Structural and functional analysis identified IPO as a member of the JRL family but with a different tetrameric association. The monomeric IPO from residues 1 to 154 shows a typical β-prism fold found in the JRL family, with 12 β-sheets (β3-β14) and 2 additional short, extended, N-terminal β-strands (β1-β2). Four IPO protomers form a compact tetrameric association by swapping their extended N termini from residues 1 to 10. Thus, the wound-inducible protein IPO from sweet potato has versatile carbohydrate binding properties and might play a role in plant defense.

IPO–Me-Man belongs to an orthorhombic space group C2221. The Matthew coefficient and solvent content for IPO–Me-Man had a reasonable value of 2.21 Å3/Da and 44.4% for 2 molecules in an asymmetric unit. Although only 2 IPO molecules were built in the IPO–Me-Man complex, the other 2 IPO molecules could be generated by symmetric operation (X, -Y, -Z) and resulted in a tetrameric association. In the structure of IPO–Me-Man, two IPO protomers were built, and only one Me-Man molecule could be observed in chain A. The temperature factor of Me-Man in the structure of IPO–Me-Man is 66.5 Å2, which is higher than that of Me-Glc, with 34.5 Å2. This phenomenon might indicate that only a few Me-Man molecules bound to IPO proteins in IPO–Me-Man, which resulted in a higher temperature factor. Nine hydrogen bonds are formed by the residues Gly21, Tyr97, Gly141, Trp142, Tyr143, and Asp145 of IPO and the atoms O1, O3, O4, O5 and O6 of Me-Man. The atom C7 of Me-Man is also involved in the Me…π interaction with Trp142 of IPO. The binding orientation of Me-Man is similar to that of Me-Glc. Me-Man and Me-Glc are epimers differing only at the C2 position, and IPO has no hydrogen bonds for C2 atom. The KA of IPO to Me-Man was the highest, 7.04×103 M−1.

>[2x]HHHHHHMALQLAAHSDARSGPVGSNGGQFWSFRPVRPLNKIVLSFSGSPDQTLNLISITFSSNPTDIITVGGVGPEPLTYTETVNIDGDIIEISGMIANYKGYNVIRSIKFTTNKKEYGPYGANAGTPFNIKIPDGNKIVGFFGNSGWYVDAIGAYYTAK> GVALGATRVIYPAGQKQVQLAVTNNDENSTYLIQSWVENADGVKDGRFIVTPPLFAMKGKKENTLRILDATNNQLPQDRESLFWMNVKAIPSMDKSKLTEN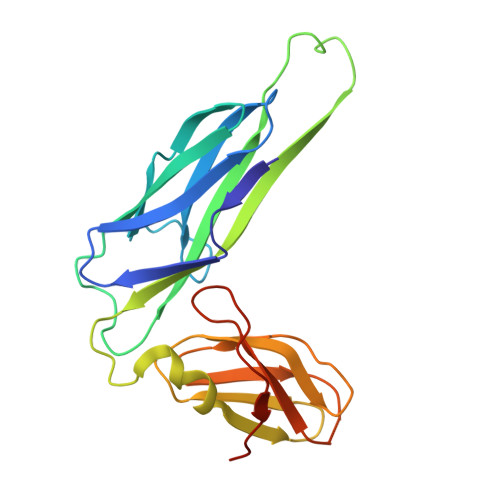TLQLAIISRIKLYYRPAKLALPPDQAAEKLRFRRSANSLTLINPTPYYLTVTELNAGTRVLENALVPPMGESAVKLPSDAGSNITYRTINDYGALTPKMTGVMEHHHHHH>MVRFLDGHTPAYDLTYNDVFVVPGRSDVASRFDVDLSTVDGSGTTIPVVVANMTAVAGRRMAETVARRGGIVVLPQDLPITAVSETVDFVKSRDLVVDTPVTLSPEDSVSDANALLHKRAHGAAVVVFEGRPIGLVTEANCAGVDRFARVRDIALSDFVTAPVGTDPREVFDLLEHAPIDVAVMTAPDGTLAGVLTRTGAIRAGIYTPAVDAKGRLRIAAAVGINGDVGAKAQALAEAGADLLVIDTAHGHQAKMLDAIKAVASLDLGLPLVAGNVVSAEGTRDLIEAGASIVKVGVGPGAMCTTRMMTGVGRPQFSAVVECAAAARQLGGHVWADGGVRHPRDVALALAAGA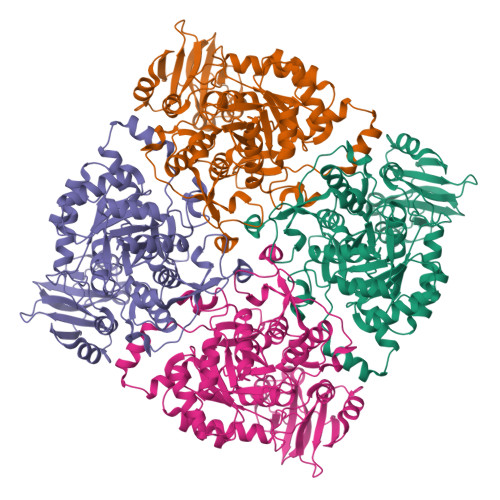SNVMIGSWFAGTYESPGDLLFDRDDRPYKESYGMASKRAVAARTAGDSSFDRARKGLFEEGISTSRMSLDPARGGVEDLLDHITSGVRSTCTYVGAANLPELHEKVVLGVQSAAGFAEGHPLPAGWTAAAKEDLEHHHHHHHH[4x]> AMADIGSEFGHRTLASTPALWASIPCPRSELRLDLVLPSAQSFRWREQSPAHWSGVLADQVWTLTQTEEQLHCTVYRGDKSQASRPTPDELEAVRKYFQLDVTLAQLYHHWGS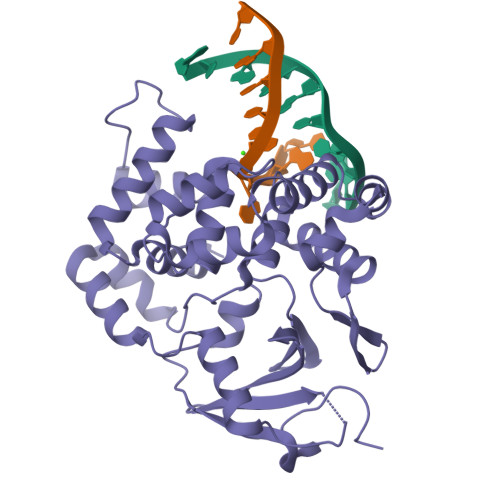VDSHFQEVAQKFQGVRLLRQDPIECLFSFICSSCNNIARITGMVERLCQAFGPRLIQLDDVTYHGFPSLQALAGPEVEAHLRKLGLGYRARYVSASARAILEEQGGLAWLQQLRESSYEEAHKALCILPGVGTQVADCICLMALDKPQAVPVDVHMWHIAQRDYSWHPTTSQAKGPSPQTNKELGNFFRSLWGPYAGWAQAVLFSADLRQSR> IKEVNQALKGHAWLKD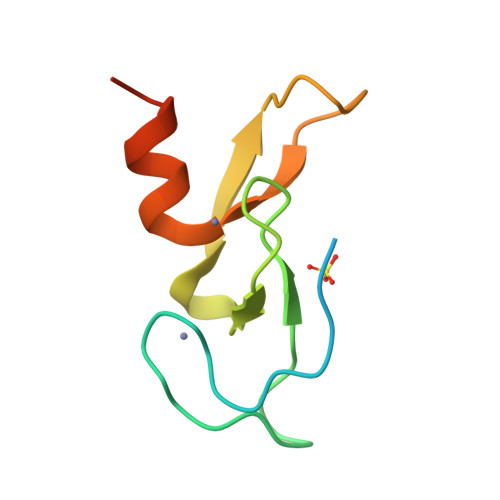DEATHCRQCEKEFSISRRKHHCRNCGHIFCNTCSSNELALPSYPKPVRVCDSCHTLLLQRCSSTAS> GSSPDKKWLGTPIEEMRRMPRCGIRLPLLRPSANHTVTIRVDLLRAGEVPKPFPTHYKDLWDNKHVKMPCSEQNLYPVEDENGERTAGSRWELIQTALLNKFTRPQNLKDAILKYNVAYSKKWDFTALIDFWDKVLEEAEAQHLYQSILPDMVKIALCLPNICTQPIPLLAAAMNHSITMSQEQIASLLANAFFCTFPRRNAKMKSEYSSYPDINFNRLFEGRSSRKPEKLKTLFCYFRRVTAAAPTGLVTFTRQSLEDFPEWERCEKPLTRLHVTYEGTIEENGQGMLQVDFANRFVGGGVTSAGLVQENIRFLINPELIISRLFTEVLDHNECLIITGTEQYSEYTGYAETYRWSRSHEDGSERDDWQRRCTEIVAIDALHFRRYLDQFVPEKMRRELNKAYCGFLR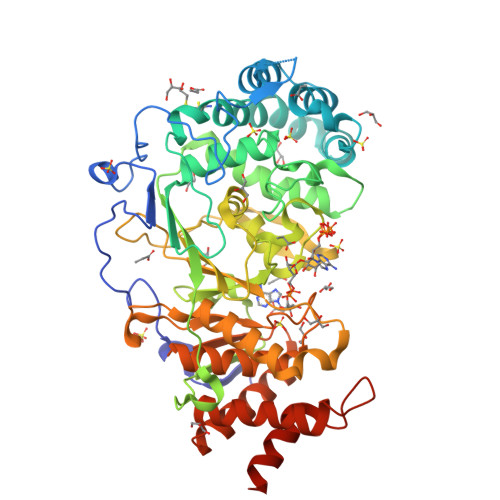PGVSSENLSAVATGNWGCGAFGGDARLKALIQILAAAAAERDVVYFTFGDSELMRDIYSMHIFLTERKLTVGDVYKLLLRYYNEECRNCSTPGPDIKLYPFIYHAVESCAETADHSGQRTGT> MTNEEPLPKKVRLSETDFKVMARDELILRWKQYEAYVQALEGKYTDLNSNDVTGLRESEEKLKQQQQESARRENILVMRLATKEQEMQECTTQIQYLKQVQQPSVAQLRSTMVDPAINLFFLKMKGELEQTKDKLEQAQNELSAWKFTPDSQTGKKLMAKCRMLIQENQELGRQLSQGRIAQLEAELALQKKYSEELKSSQDELNDFIIQLDEEVEGMQST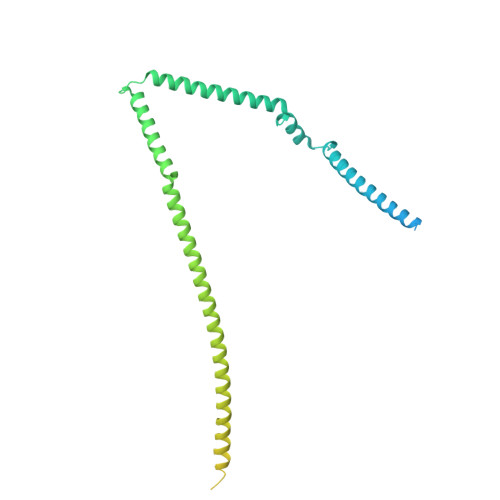ILVLQQQLKETRQQLAQYQQQQSQASAPSTSRTTASEPVEQSEATSKDCSRLTNGPSNGSSSRQRTSGSGFHREGNTTEDDFPSSPGNGNKSSNSSEERTGRGGSGYVNQLSAGYESVDSPTGSENSLTHQSNDTDSSHDPQEEKAVSGKGNRTVGSRHVQNGLDSSVNVQGSVL> LIPVSLVDLININIIFYILLLYTLLL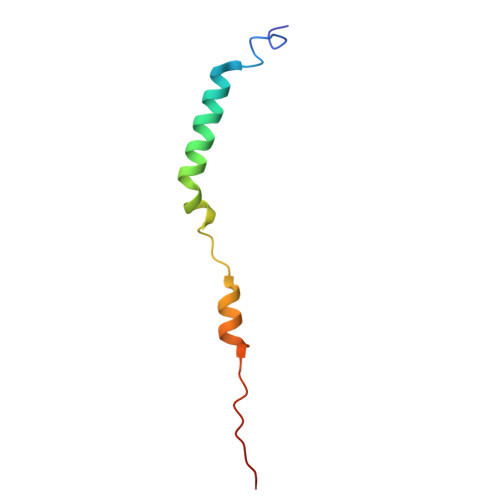FFIPLFLASINYTYHYIYKYYNYNYNFINNN>[2x]GSYSKFWPKGGLPGILHHYTETLVTFEYTTTTTRKPHSLLFVGGLGDGLATTSYLADLAHALQPTEWSLFTLTLTSSYQSWGLGHLDRDTNEIAQCLKYIKEYKTEKFGGSASSGKIVLMGHSTGSQCVLHYLSRPNPHTHTPAFDPYLEHVERMPLDGAIMQAPVSDREAIQWVLAEGLGDRTPAEIRPVFEKLTSMAREAARDADAGTDV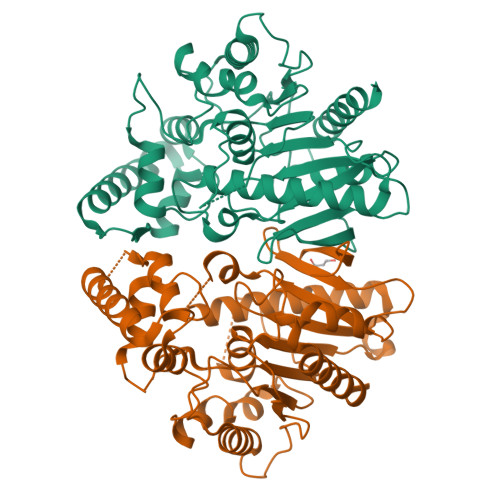LLPLAMTSLVYPAHTPLSARRFLSLTSPESPESPSEDDLFSSDLSDEQLGKTFGMIREQGLLRGKLMVLFSGADQSVPAWVDKDTLLSRWRNATDHNGEAAIWDENSGIIPNASHALSNDDQAEPRNFLVNKVLGYLSALVKA3-oxo-3,4-dihydro-2H-1,4-benzothiazine-7-carboxylic acid | C9 H7 N O3 S | 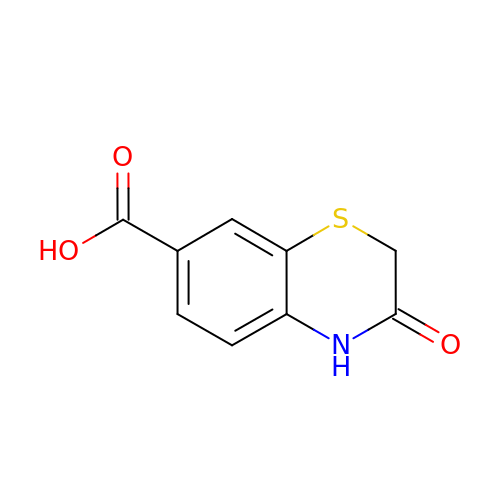PMIQHWMFUZMWOX-UHFFFAOYSA-N Galactosaminogalactan (GAG), an α-1,4-linked linear exopolysaccharide of galactose (Gal) and N-acetylgalactosamine (GalNAc), is essential for A. fumigatus biofilm formation and a key virulence factor. Lastly, GAG is partially deacetylated by the secreted protein Agd3 and deletion of agd3 abolishes this modification. Herein, we show that A. fumigatus Agd3 has a unique three-domain architecture and that the enzyme specifically deacetylates α-1,4-GalNAc oligosaccharides in a metal-dependent manner. Agd3 has a novel carbohydrate-binding module (CBM) that extends the substrate binding groove, increases activity on soluble GAG, and influences the location of deacetylation within oligosaccharides.

To gain insights into the function of Agd3, structural studies of the predicted globular protein, residues 141–806, were pursued. Agd3 crystallized in the hexagonal space group P 61 2 2. Diffraction data were anisotropic with diffraction limits of 2.6 Å in one dimension and 3 Å in the other two dimensions. The structure was solved by Zn single-wavelength anomalous dispersion and refined to Rwork and Rfree of 19% and 24%, respectively. Agd3 has a unique compact three-domain structure. The N-terminal domain, comprising residues 141–364, adopts a mixed α/β/α-fold (α/β/α-domain) with a seven-stranded β-sheet at its center. The central domain, residues 365–733, contains the CE4 homology region and has a distorted (β/α)7-fold (CE-domain). The C-terminal domain spanning residues 733–806 forms six β-strands in a seven-stranded β-sandwich. The N- and C-terminal domains increase the stability of the CE-domain, as constructs lacking one or both of these accessory domains expressed poorly and could not be purified to homogeneity from either E. coli or Pichia pastoris. Mapping surface conservation reveals a highly conserved electronegative cleft in the CE-domain. IcaB has only 5.2% sequence identity to Agd3 and aligned poorly compared with the other CE4 enzymes with a RMSD of 3.80 Å over 134 α-carbons. The catalytic cations of these CE4 enzymes overlapped with a Zn ion in Agd3, suggesting that Agd3 is also metal dependent.

> MGSSHHHHHHSSGLVPRGSHGSVLSNILVIAKDSSAASSATSGLNAYGIPYTTLLVPQAGVGLPALNSSNVGNYGGIVVAAEVSYDYGGTTGYQSALTTDQWNQLYAYQLEYGVRMVQFDVYPGPKFGASAVNGGCCNTGVEQLLSFTDTSDFPTAGLKTGATVSTEGLWHYPATISNSSNTKEIAQFAPNAVTSTASTAAVINNFDGREQMAFFIGFATDWSATSNYLQHAWITWLTRGLYAGHRRVNLNTQIDDMFLVTDIYYPNGSTFRITVEDMNGISAWVPTINAKMNPGSSYFVEVGHNGNGNIEQSSSTDAGAAACNGGGIEYDSPPDTPLEFKKPLGTGTDLWPSTPTTYDWTVACTQLDDLLRWWTTPANRDAFGHISHTFTHEEQNNATYADVFKEISFNQAWLKQVGLDQAKWFTSNGIIPPAITGLHNGDALQAWWDNGIRNCVGDNTRPVLMNQQNAMWPYFTTVESDGFAGMQVNPRWATRIYYNCDTPACTVQEWIDTSAGAGSFDDLLAVEKADTMRHLLGLRHDGYMFHQANLRNADVTPITVNGVTAKYSIFQAWVETIVQEFVRLVDWPLVTITHQEMSENFLARYQRDQCGYGLSYAVADKKITAVTVTATGNTCSRPIPVTFPVAPTSTQGYATEQLGSDPLTVWVQLSGSPVTFTLSTPIAL>GSGSGSCVKWFIYGVIAVYICYTLIVHKRYQEKEELTSSVRVTLKGVAHVDRIWDAAEYTIPTQTRDSFFVMTNIIRTENQIQKTCPEYPTAKAICSSDKSCAKGIVDVHSNGVQTGKCVHYNITHKTCEIKAWCPVQGEERPPVPAVLRSSEDFTVFIKNNIHFPTFQYTVQNISPKLNTSCKFNKVTAPLCPIFRLGDILQEAKENFSEMAVKGGIIAIEIKWDCDLDSWSYYCSPEYSFRRLDDKTRTQYPGFSIRFARHYKLP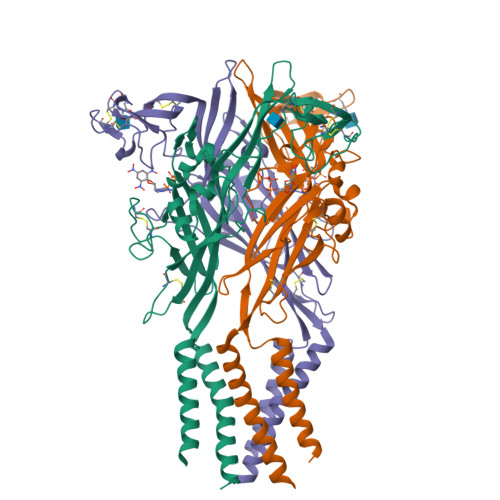DGTEQRTLFKAYGIRFDVLVFGMGGQFKLIELFTFIGSTIAYFGLAVTIIEMCFHLYNLE[3x]> MVSTQNEPHRFPPDFQWGVATSSYQIEGAVEADGRSPSIWDTFCARPGAIADGSTGAIANDHYHRYREDIAIMKQLGVNAYRFSIAWPRILPDGRGRVNQAGVDFYERLVDSLLEQGIEPYATLYHWDMPQVQHDRTPWYDRGVVDAFVEYTDV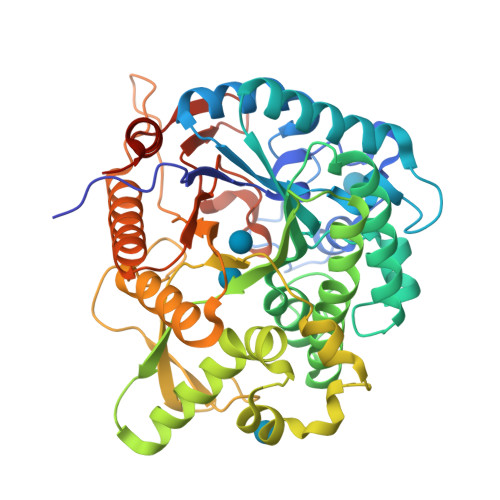ITRRLSDRVKYWMTLNEPWVISFLGYGAGEHAPGLRDKELYLRAAHHVLLAHGKAMPVIRANGNAQTKAGIVLNLNWVNAASDSPEDQAAARRYDQFFNRWFAEPLYNGRYPEELLEWYGRDLVPVQPGDFDIITTPTDFLAVNYYARTTVKAGSTDPMLQVDFVRPPGEYTAMDWEVYPQGLYNILNWLHTDYAPPALYVTENGAAYDDQVSAAGEVDDPQRLAYLEGHFEAAYRAIQAGIPLKGYFVWSLMDNFEWGRGFEKRFGIVFVDYATQQRIIKRSGKWFSQVTRANGLPAPQTTL Cyclic GMP-dependent protein kinases (PKGs) are key mediators of the nitric oxide/cyclic guanosine monophosphate (cGMP) signaling pathway that regulates biological functions as diverse as smooth muscle contraction, cardiac function, and axon guidance. PKGs belong to the AGC family of protein kinases and have N-terminal regulatory (R) and C-terminal catalytic (C) domains. The R-domain comprises a leucine zipper (LZ) domain, a linker region with an auto-inhibitory (AI) sequence, and two cyclic nucleotide-binding (CNB-A and -B) domains. By analogy to PKA, the PKG R-domain is thought to bind via its AI sequence to the C-domain active site to form an auto-inhibited R:C state; binding of cGMP to the R-domain destabilizes this state and allows active kinase to phosphorylate downstream substrates.

A mutation that causes familial Thoracic Aortic Aneurysms and Dissections (TAAD) maps to this arginine of CNB-A (PKG Iα residue 177), and the mutation to glutamine constitutively activates the enzyme. Mutation R177Q in PKG Iα is associated with TAAD and constitutively activates the holoenzyme despite weakening cGMP affinity for CNB-A more than 105-fold. We also present a high-resolution structure of the CNB-A domain with the TAAD mutation, which reveals a closed cGMP pocket. The similarity of this mutant domain to wildtype cGMP-bound structures and its differences with the open pocket in the AI enzyme explain the constitutive activation of the holoenzyme in TAAD. Since the RQ mutation does not alter folding or prevent adoption of the closed conformation, we propose that the CNB-A sequence is biased to adopt the closed state. Because the PBC of the RQ CNB-A domain makes intermonomer crystal contacts, it is possible that these contacts help stabilize the closed state. We conclude that neither crystal contacts nor interactions with cGMP are needed to drive either the wildtype or mutant domain to the closed state, supporting our hypothesis that PBC-A is biased toward the closed state. Chemical shifts of apo R192Q NH resonances are more similar to those of the cGMP-bound wildtype than to the apo wildtype, consistent with the mutation inducing a similar conformational change as cGMP binding to wildtype. We therefore conclude that the RQ mutation causes constitutive kinase activation by allowing CNB-A to adopt a closed PBC-A similar to that of cGMP-bound wildtype without binding cGMP. The activating effect of the CNB-A RQ mutation reflects destabilization of the auto-inhibited state we describe here.

>QAFRKFTKSERSKDLIKEAILDNDFMKNLELSQIQEIVDCMYPVEYGKDSCIIKEGDVGSLVYVMEDGKVEVTKEGVKLCTMGPGKVFGELAILYNCTQTATVKTLVNVKLWAIDRQCFQTIMMRTGLIKHTEY[2x]> GGDVITQDTKQLPLTARNFINQYFSKPHISHIKIESEILQTKKYEVLLTDRTEIDFDKKGNWLEVDCKKSAVPEALIPVPVKEYVKANFPREIITKIERGRTGVEIELGNDYSLKFNKKGKFVSM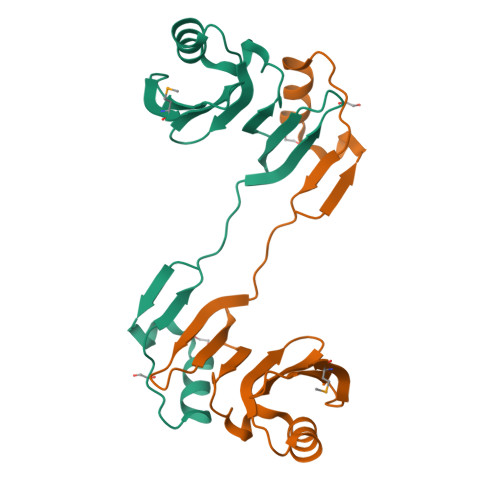DD2-[1-[(3-bromophenyl)methyl]-2-methyl-3-oxamoyl-indol-4-yl]oxyethanoic acid | C20 H17 Br N2 O5 | 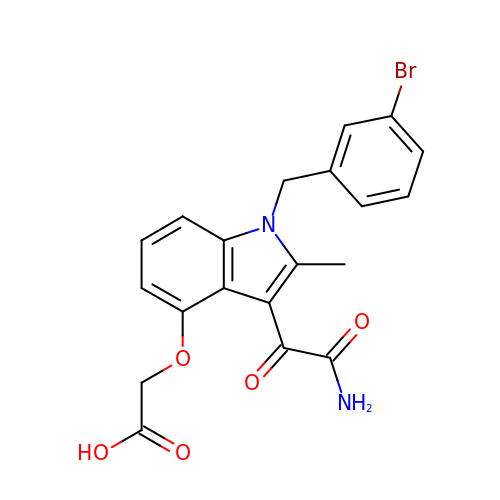ZWWWBZCFNLMLRT-UHFFFAOYSA-N> SLHMIDYKEIEVEEVVGRGAFGVVCKAKWRAKDVAIKQIESESERKAFIVELRQLSRVNHPNIVKLYGACLNPVCLVMEYAEGGSLYNVLHGAEPLPYYTAAHAMSWCLQCSQGVAYLHSMQPKALIHRDLKPPNLLLVAGGTVLKICDFGTACDIQTHMTNNKGSAAWMAPEVFEGSNYSEKCDVFSWGIILWEVITRRKPFDEIGGPAFRIMWAVHNGTRPPLIKNLPKPIESLMTRCWSKDPSQRPS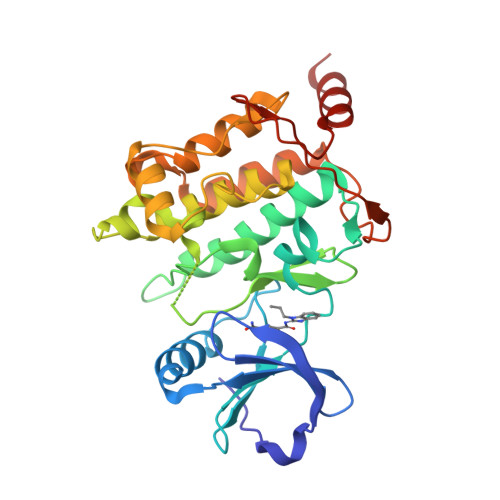MEEIVKIMTHLMRYFPGADEPLQYPCQHSLPPGEDGRVEPYVDFAEFYRLWSVDHGE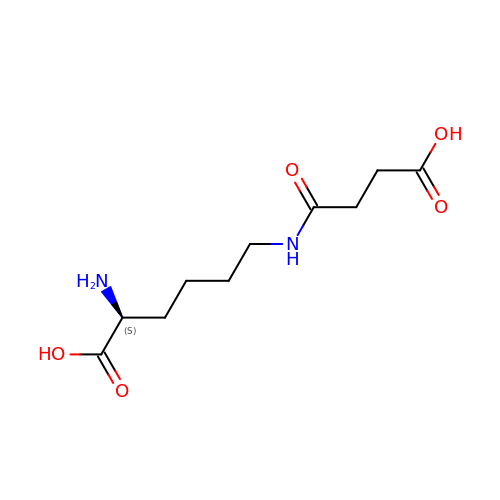(2S)-2-azanyl-6-[(4-hydroxy-4-oxo-butanoyl)amino]hexanoic acid | C10 H18 N2 O5 | ZAFOVBXOMIXMTH-ZETCQYMHSA-N(3R)-N-(4-CHLOROPHENYL)-3-(HYDROXYMETHYL)-1,2,3,4-TETRAHYDROISOQUINOLINE-7-SULFONAMIDE 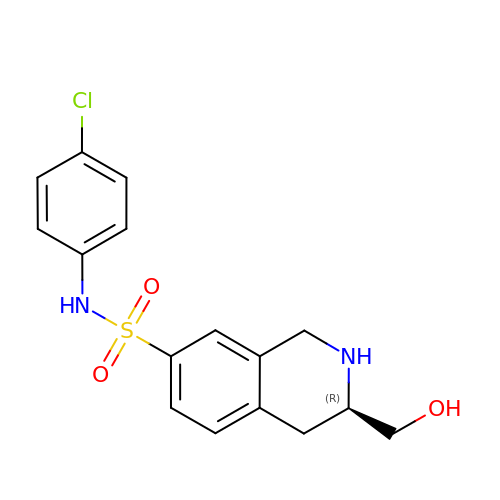| C16 H17 Cl N2 O3 S | YTBGBMPLINFTBQ-OAHLLOKOSA-N> MASHKLLVTPPKALLKPLSIPNQLLLGPGPSNLP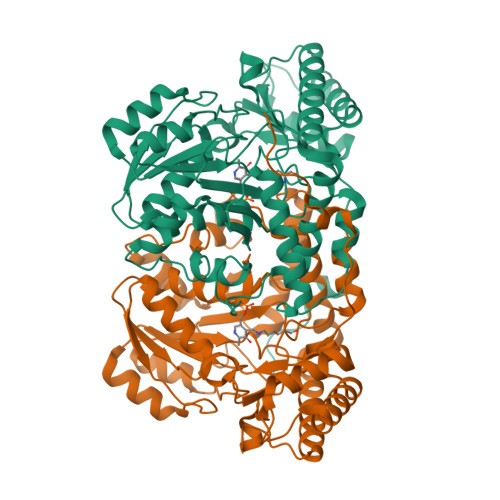PRIMAAGGLQMIGSMSKDMYQIMDEIKEGIQYVFQTRNPLTLVISGSGHCALEAALVNVLEPGDSFLVGANGIWGQRAVDIGERIGARVHPMTKDPGGHYTLQEVEEGLAQHKPVLLFLTHGESSTGVLQPLDGFGELCHRYKCLLLVDSVASLGGTPLYMDRQGIDILYSGSQKALNAPPGTSLISFSDKAKKKMYSRKTKPFSFYLDIKWLANFWGCDDQPRMYHHTIPVISLYSLRESLALIAEQGLENSWRQHREAAAYLHGRLQALGLQLFVKDPALRLPTVTTVAVPAGYDWRDIVSYVIDHFDIEIMGGLGPSTGKVLRIGLLGCNATRENVDRVTEALRAALQHCPKKKL>MAHHHHHHHRSGKLTGKTALVTGSSRGIGRATAIRLAREGALVAVHCSRNREAADETVA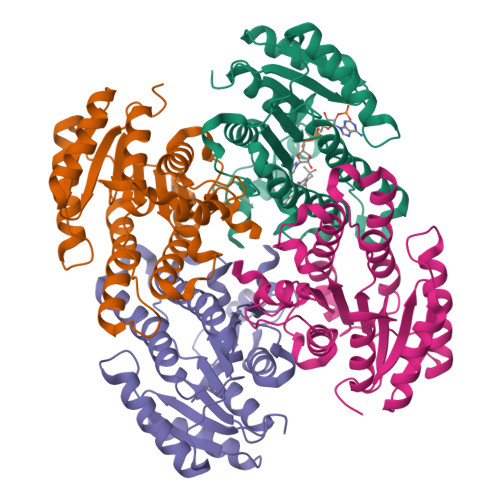TIEKEGGRAFSVLAELGVPGDVHELFLALERGLKERTDATTLDILVNNAGVMGGVAPEEVTPELFDRLVAVNAKAPFFIVQRALTLIPDGGRIINISSGLTRFANPQEVAYAMTKGAMDQLTLHFAKHLGSRNITVNSVGPGITNNGTPVFDNPEAVAQMAGYSVFNRVGEVTDVADVVAFLAGDDARWITGSYLDASGGTLLG[4x]>MDAESIEWKLTANLRNGPTFFQPLADSIEPLQFKLIGSDTVATAFPVFDTKYIPDSLINYLFKLFNLEIESGKTYPQLHSLTKQGFLNYWFHSFAVVVLQTDEKFIQDNQDWNSVLLGTFYIKPNYAPRCSHNCNAGFLVNGAHRGQKVGYRLAQVYLNWAPLLGYKYSIFNLVFVTNQASWKIWDKLNFQRIGLVPHAGILNGFSE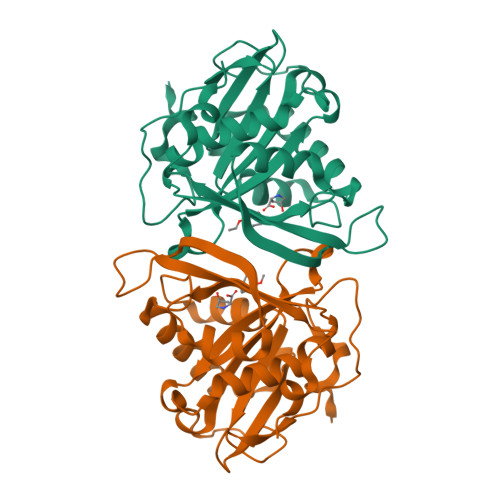PVDAIIYGKDLTKIEPEFLSME[12x]> QQIGTYTAETHPSLSWSTCKSGGSCTTNSGAITLDANWRWVHGVNTSTNCYTGNTWNSAICDTDASCAQDCALDGADYSGTYGITTSGNSLRLNFVTGSNVGSRTYLMADNTHYQIFDLLNQEFTFTVDVSHLPCGLNGALYFVTMDADGGVSKYPNNKAGAQYGVGYCDSQCPR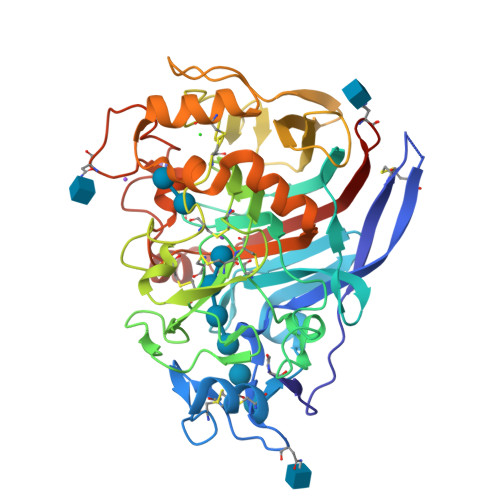DLKFIAGQANVEGWTPSANNANTGIGNHGACCAELDIWEANSISEALTPHPCDTPGLSVCTTDACGGTYSSDRYAGTCDPDGCDFNPYRLGVTDFYGSGKTVDTTKPFTVVTQFVTNDGTSTGSLSEIRRYYVQNGVVIPQPSSKISGISGNVINSDYCAAEISTFGGTASFSKHGGLTNMAAGMEAGMVLVMSLWDDYAVNMLWLDSTYPTNATGTPGAARGTCATTSGDPKTVESQSGSSYVTFSDIRVGPFNSTFSGG>TAAVGADLLGDGRPETLWLGIGTLLMLIGTFYFIVKGWGVTDKEAREYYSITILVPGIASAAYLSMFFGIGLTEVQVGSEMLDIYYARYADWLFTTPLLLLDLALLAKVDRVSIGTLVGVDALMIVTGLVGALSHTPLARYTWWLFSTICMIVVLYFLATSLRAAAKERGPEVASTFNTLTALVLVLWTAYPILWII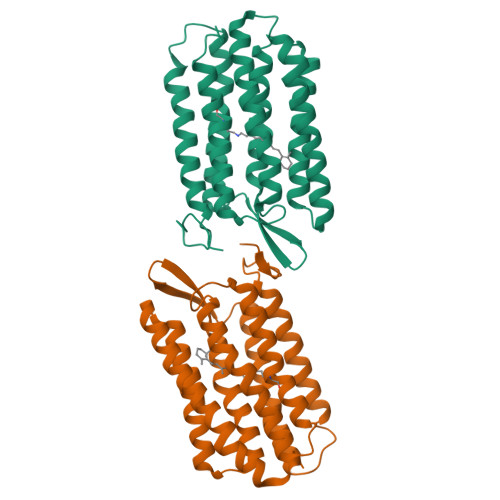GTEGAGVVGLGIETLLFMVLDVTAKVGFGFILLRSRAILGDTEAPEPSAGAEASAAD[2x]Herpesvirus-associated ubiquitin-specific protease (HAUSP, also known as USP7), a deubiquitylating enzyme of the ubiquitin-specific processing protease family, specifically deubiquitylates both p53 and MDM2, hence playing an important yet enigmatic role in the p53–MDM2 pathway. Here we demonstrate that both p53 and MDM2 specifically recognize the N-terminal tumor necrosis factor–receptor associated factor (TRAF)–like domain of HAUSP in a mutually exclusive manner. The crystal structures of the HAUSP TRAF-like domain in complex with p53 and MDM2 peptides, determined at 2.3-Å and 1.7-Å resolutions, respectively, reveal that the MDM2 peptide recognizes the same surface groove in HAUSP as that recognized by p53 but mediates more extensive interactions. Structure-based sequence alignment of the three HAUSP-binding peptides revealed a conserved four-residue binding motif with the consensus sequence of (Ø/E)-G-(Ø/G)-S, where Ø denotes a non-polar residue.

To investigate this process, we sought to determine the crystal structure of a larger HAUSP fragment (residues 53–560), which contains both the substrate-binding TRAF-like domain and the catalytic core domain. We succeeded in the generation of crystals for this HAUSP fragment and solved its structure at 3.2 Å-resolution. The structure contains two well-ordered domains, the TRAF-like domain as a β-sandwich and the isopeptidase domain as a tripartite architecture. Interestingly, there is very limited interaction between these two domains, and the intervening linker sequences (residues 199–206) have high-temperature factors in the crystals, suggesting that the substrate-binding domain is coupled to the catalytic domain through a relatively flexible linker sequence. In addition, the ubiquitin-binding pocket of the catalytic core domain and the substrate-binding groove of the TRAF-like domain are located on the same side of the molecule. On the basis of the structure and previous information about ubiquitin binding, we modeled how HAUSP may recognize an ubiquitylated MDM2 molecule. A conjugated ubiquitin moiety is bound by the Fingers domain of HAUSP, with the C-terminus of ubiquitin docked in the active-site cleft between the Palm and the Thumb. The close proximity of the C-terminus of HAUSP-bound ubiquitin and the MDM2 peptide suggests that HAUSP likely prefers to cleave the ubiquitin chain at the proximal end of the ubiquitylated MDM2. Second, the linker sequence between the TRAF-like domain and the catalytic domain is flexible, which allows some lateral movement between these two domains and hence enhanced access to multiple ubiquitylation sites within the same substrate.

>GSHMNGNVALSDGHNTAEEDMEDDTSWRSEATFQFTVERFSRLSESVLSPPCFVRNLPWKIMVMPRFYPDRPHQKSVGFFLQCNAESDSTSWSCHAQAVLKIINYRDDEKSFSRRISHLFFHKENDWGFSNFMAWSEVTDPEKGFIDDDKVTFEVFVQADAPHGVAWDSKKHTGYVGLKNQGATCYMNSLLQTLFFTNQLRKAVYMMPTEGDDSSKSVPLALQRVFYELQHSDKPVGTKKLTKSFGWETLDSFMQHDVQELCRVLLDNVENKMKGTCVEGTIPKLFRGKMVSYIQCKEVDYRSDRREDYYDIQLSIKGKKNIFESFVDYVAVEQLDGDNKYDAGEHGLQEAEKGVKFLTLPPVLHLQLMRFMYDPQTDQNIKINDRFEFPEQLPLDEFLQKTDPKDPANYILHAVLVHSGDNHGGHYVVYLNPKGDGKWCKFDDDVVSRCTKEEAIEHNYGGHDDDLSVRHCTNAYMLVYIRESKLSEVLQAVTDHDIPQQLVERLQEEKRIEAQKRKERQE[2x]> MTQAEIKLCSLLLQEHFGEIVEKIGVHLIRTGSQPLRVIAHDTGTSLDQVKKALCVLVQHNLVSYQVHKRGVVEYEAQCSRVLRMLRYPRYIYTTKTLYSDTGELIVEELLLNGKLTMSAVVKKVADRLTETMEDGKTMDYAEVSNTFVRLADTHFVQRCPSVPTTENSDPGPPPPAPTLVINEKDMYLVPKLSLIGKGKRRRSSDEDAAGEPKAKRPKYTTDNKEPIPDDGIYWQANLDRFHQHFRDQAIVSAVANRMDQTSSEIVRTMLRMSEITTSSSAPFTQPLSSNEIFRSLPVGYNISKQVLDQYLTLLADDPLEFVGKSGDSGGGMYVINLH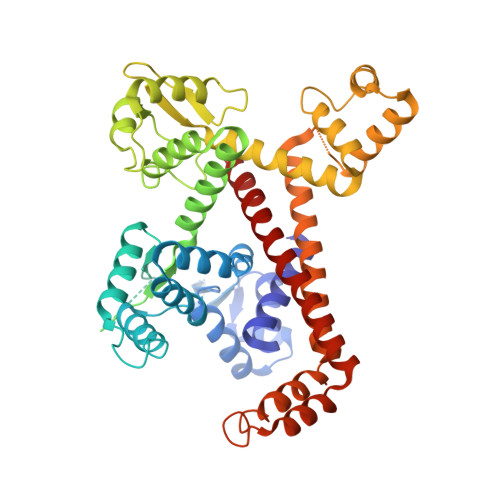KALASLATATLESVVQERFGSRCARIFRLVLQKKHIEQKQVEDFAMIPAKEAKDMLYKMLSENFMSLQEIPKTPDHAPSRTFYLYTVNILSAARMLLHRCYKSIANLIERRQFETKENKRLLEKSQRVEAIIASMQATGAEEAQLQEIEEMITAPERQQLETLKRNVNKLDASEIQVDETIFLLESYIECTMKRQ> MEFVAKLFKFFKDLL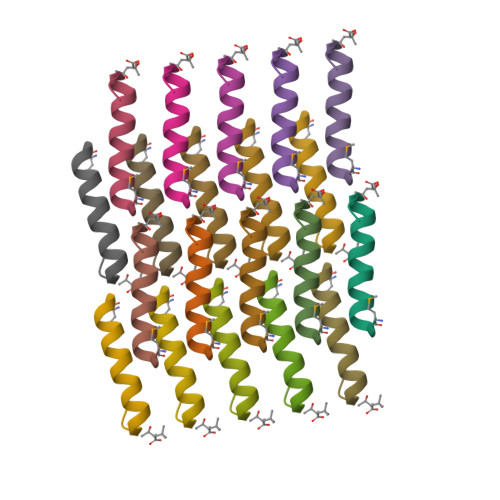GKFLGNN>MQKPVCLVVAMTPKRGIGINNGLPWPHLTTDFKHFSRVTKTTPEEASRFNAVVMGRKT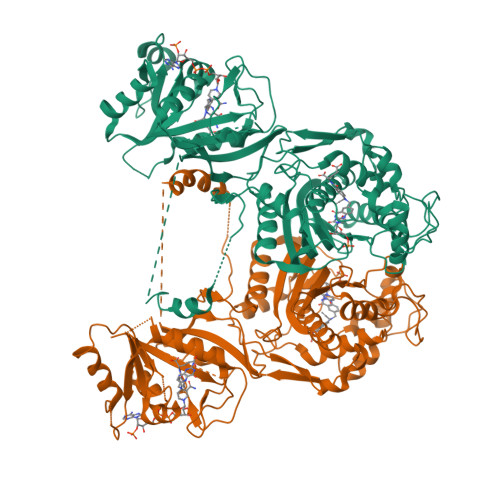WESMPRKFRPLVDRLNIVVSSSLKEEDIAAEKPQAEGQQRVRVCASLPAALSLLEEEYKDSVDQIFVVGGAGLYEAALSLGVASHLYITRVAREFPCDVFFPAFPGDDILSNKSTAAEKDNEATYRPIFISKTFSDNGVPYDFVVLEKRRKTDDAATAEPSNAMSSLTSTRETTPVHGLQAPSSAAAIAPVLAWMDEEDRKKREQKELIRAVPHVHFRGHEEFQYLDLIADIINNGRTMDDRTGVGVISKFGCTMRYSLDQAFPLLTTKRVFWKGVLEELLWFIRGDTNANHLSEKGVKIWDKNVTREFLDSRNLPHREVGDIGPGYGFQWRHFGAAYKDMHTDYTGQGVDQLKNVIQMLRTNPTDRRMLMTAWNPAALDEMALPPCHLLCQFYVNDQKELSCIMYQRSCDVGLGVPFNIASYSLLTLMVAHVCNLKPKEFIHFMGNTHVYTNHVEALKEQLRREPRPFPIVNILNKERIKEIDDFTAEDFEVVGYVPHGRIQMEMAV[8x]> MNIPKPADSTWTDDQWNAIVSTGQDILVAAAAGSGKTAVLVERMIRKITAEENPIDVDRLLVVTFTNASAAEMKHRIAEALEKELVQRPGSLHIRRQLSLLNRASISTLHSFCLQVLKKYYYLIDLDPGFRIADQTEGELIGDEVLDELFEDEYAKGEKAFFELVDRYTTDRHDLDLQFLVKQVYEYSRSHPNPEAWLESFVHLYDVSEKSAIEELPFYQYVKEDIAMVLNGAKEKLLRALELTKAPGGPAPRADNFLDDLAQIDELIQHQDDFSELYKRVPAVSFKRAKAVKGDEFDPALLDEATDLRNGAKKLLEKLKTDYFTRSPEQHLKSLAEMKPVIETLVQLVISYGKRFEAAKQEKSIIDFSDLEHYCLAILTAENDKGEREPSEAARFYQEQFHEVLVDEYQDTNLVQESILQLVTSGPEETGNLFMVGDVKQSIYRFRLAEPLLFLSKYKRFTESGEGTGRKIDLNKNFRSRADILDSTNFLFKQLMGGKIGEVDYDEQAELKLGAAYPDNDETETELLLIDNAEDTDASEEAEELETVQFEAKAIAKEIRKLISSPFKVYDGKKKTHRNIQYRDIVILLRSMPWAPQIMEELRAQGIPVYANLTSGYFEAVEVAVALSVLKVIDNPYQDIPLASVLRSPIVGADENELSLIRLENKKAPYYEAMKDYLAAGDRSDELYQKLNTFYGHLQKWRAFSKNHSVSELIWEVYRDTKYMDYVGGMPGGKQRQANLRVLYDRARQYESTAFRGLFRFLRFIERMQERGDDLGTARGLSEQEDVVRLMTIHSSKGLEFPVVFVAGLGRNFNMMDLNKSYLLDKELGFGTKYIHPQLRISYPTLPLIAMKKKMRRELLSEELRVLYVALTRAKEKLFLIGSCKDHQKQLAKWQASASQTDWLLPEFDRYQARTYLDFIGPALARHRDLGDLAGVPAHADISGHPARFAVQMIHSYDLLDDDLEERMEEKSERLEAIRRGEPVPGSFAFDEKAREQLSWTYPHQEVTQIRTKQSVSEIKRKREYEDEYSGRAPVKPADGSILYRRPAFMMKKGLTAAEKGTAMHTVMQHIPLSHVPSIEEAEQTVHRLYEKELLTEEQKDAIDIEEIVQFFHTEIGGQLIGAKWKDREIPFSLALPAKEIYPDAHEADEPLLVQGIIDCLYETEDGLYLLAYKSDRIEGKFQHGFEGAAPILKKRYETQIQLYTKAVEQIAKTKVKGCALYFFDGGHILTL;> MGAEFLVGRSGSGKTKLIINSIQDELRRAPFGKPIIFLVPDQMTFLMEYELAKTPDMGGMIRAQVFSFSRLAWRVLQHT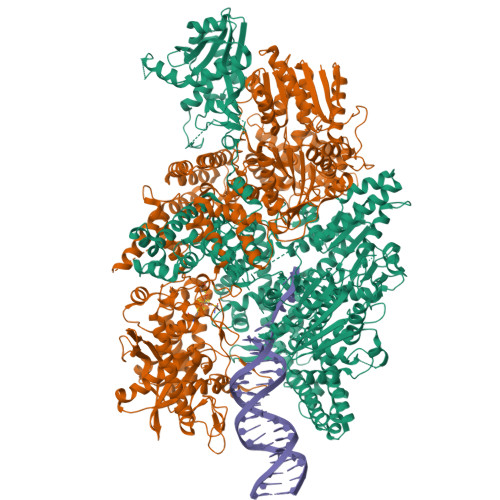GGMSRPFLTSTGVQMLLRKLIEEHKQEFKVYQKASDKSGFTAQVERMLTEFKRYCLEPEDIRRMAESGTASEYRGERVLSEKLHDLSILYQQMEKSLADQYLHSEDYLTLLAEHIPLAEDIKGAHIYVDGFYQFTPQEFRVLEQLMVHAEHITFSLTADKPSYEREPHELELFRMTGKTYYRLHQKAKELNLDITYKELSGTERHTKTPELAHLEAQYEARPAIPYAEKQEALTVMQAANRRAELEGIAREIHALVREKGYRYKDVAILARQPEDYKDMVKEVFADYEIPYFIDGKASMLNHPLIEFIRSSLDVLKGNWRYEAVFRCVKTELLFPLNEPKAKVREQVDQLENYCIAYGIKGDRWTKGDRFQYRRFVSLDDDFAQTDQEIEMENMLNDTRDWIVPPLFQLQKRMKKAKTVQEKAEALYRYLEETDVPLKLDQERQRAEDDGRIIEAQQHQQAWDAVIQLLEEFVEMMGDDEISLDLFQQMIEAGAESLTFSLIPPALDQVFVGNMDLSRMYGTSCTFVLGANDGVLPARPDENGVLSDDDREWLKTIGVELSSGGRERLLDEHFLIYMAFSSPSDRLYVSYPIADAEGKTLLPSMIVKRLEELFPHHKERLLTNEPEQVSDEEQLMYVVNKSVAQSFTASQLRLWTREYDISDVWWSTYNVLMSEQDRLQSKKLFSSLFFRNEVKQLERSVSRQLYGERIQGSVSRMETFNACPFSHFASHGLHLKERQFFKLEAPDIGQLFHSSLKLISDRLRDEKLDWRDLTKEQCELFSYDAVERLAPKLQKEILLSSNRHYYVKEKLQKIVTRVSGILSEHAKASGFVPIGLELGFGGKGPLPPLTFQLKNGCTMELVGRIDRVDKAESSKGLLLRIVAYKSSDKGLDLAEVYYGLALQMLTYLDLSITHSADWLGMRATPAGVLYFHIHDPMIQSNLPLGLDEIEQEIFKKFKMKGLLLGDQEVVRLMDTTLQEGRSNIINAGLKKDGSLRSDSAAVGEKEFDLLTKHVRRTFQEAGEQITDGRVSIEPYKMKNKTPCTYCAFKSVCQFDESLEENEYRPLKAEKDKTILEWIKKEADGNEHS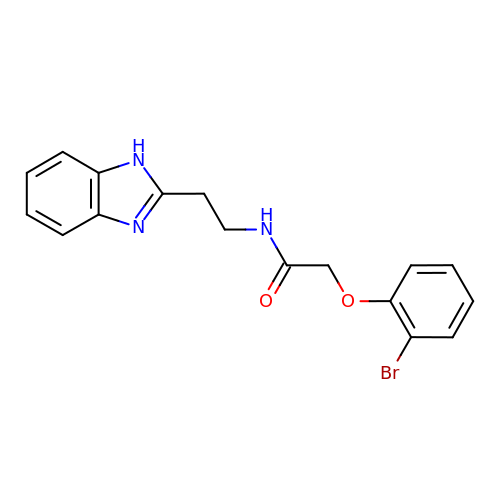N-[2-(1H-benzimidazol-2-yl)ethyl]-2-(2-bromophenoxy)acetamide | C17 H16 Br N3 O2 | XWFRNTHGPRGCNS-UHFFFAOYSA-N>PTFPIDSGARIGEMKRVTKETNVSVKINLDGTGVADNSSGIPFLDHMLDQLASHGLFDVHVKATGDTHIDDHHTNEDVALAIGTALLQALGDRKGINRFGNFSAPLDEALVHVSLDLSGRPHLGYDLNIPTQRVGKYDTQLVEHFFQSLVNTSGMTLHIRQFSGTNSHHIIEATFKAFARALRQATEYDTRRRGTIPSSKGVLSRS[8x]

Plant HISN5 catalyzes the sixth step of the HBP, in which imidazole-glycerol phosphate (IGP) is dehydrated to form imidazole-acetol phosphate (IAP). The MtHISN5 subunit contains a four α-helix bundle sandwiched between two β-sheets whose four strands are almost perpendicular to each other. In solution, MtHISN5 forms a homo 24-mer with octahedral (432) symmetry of approx. 110 Å diameter and a total mass of 540 kDa. The dimensions of the MtHISN5 oligomer did not change significantly after the binding of IG2, indicating a lack of major conformational rearrangements. The active site of MtHISN5 (see below) contains two Mn2+ cations (Mn1 and Mn2) bound by residues belonging to different subunits.

The crystal structure at 1.55 Å was obtained in space group R3 and comprises eight chains in the asymmetric unit (ASU). The crystal structures cover the MtHISN5 sequence starting from Gly77 or Ala78 through Arg260/261 (chain and structure-dependent). The crystal structure at 1.55 Å resolution contains imidazole (IMD), sodium ion, chloride ion, formate (FMT), 1,2-ethanediol (EDO), glycerol (GOL), and tris(hydroxymethyl) aminomethane (TRS). The crystal structures were obtained in the presence of formate (FMT) between Mn1 and Mn2, which completes their coordination spheres. FMTs primary location was in the active sites, between Mn1 and Mn2. However, it was very interesting to find that IMD (IMD1) bound not between the Mn2+ ions in the active site, but instead was positioned approximately 3.8 Å from the C atom of FMT. In MtHISN5, IMD1 forms hydrogen bonds with FMT and water. The fact that we see FMT between Mn2+ and imidazole positioned differently suggests that the bi-Mn2+ cluster has a high affinity for carboxylate, in addition to the imidazole of IGP or IAP. We postulate that the carboxylate and imidazole binding sites can be used as pharmacophores for the design of selective inhibitors of plant HISN5. Consistently, we identified TRS (121 Da) and CIT (192 Da) in the 3- and 4-fold tunnels, respectively.> EPGDGAQTWARFSRPPAPEAAGLFQGTFPDGFLWAVGSAAYQTEGGWQQHGKGASIWDTFTHHPLAPPGDSRNASLPLGAPSPLQPATGDVASDSYNNVFRDTEALRELGVTHYRFSISWARVLPNGSAGVPNREGLRYYRRLLERLRELGVQPVVTLYHWDLPQRLQDAYGGWANRALADHFRDYAELCFRHFGGQVKYWITIDNPYVVAWHGYATGRLAPGIRGSPRLGYLVAHNLLLAHAKVWHLYNTSFRPTQGGQVSIALSSHWINPRRMTDHSIKECQKSLDFVLGWFAKPVFIDGDYPESMKNNLSSILPDFTESEKKFIKGTADFFALCFGPTLSFQLLDPHMKFRQLESPNLRQLLSWIDLEFNHPQIFIVENGWFVSGTTKRDDAKYMYYLKKFIMETLKAIKLDGVDVIGYTAWSLMDGFEWHRGYSIRRGLFYVDFLSQDKMLLPKSSALFYQKLIEKNGFPPLPENQPLEGTFPCDFAWGVVDNYIQVDTTLSQFTDLNVYLWDVHHSKRLIKVDGVVTKKRKSYCVDFAAIQPQIALLQEMHVTHFRFSLDWALILPLGNQSQVNHTILQYYRC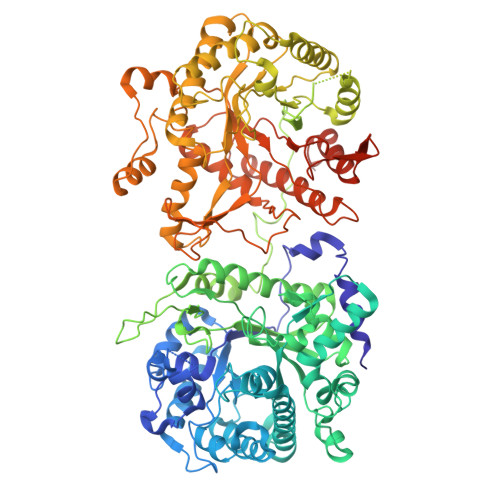MASELVRVNITPVVALWQPMAPNQGLPRLLARQGAWENPYTALAFAEYARLCFQELGHHVKLWITMNEPYTRNMTYSAGHNLLKAHALAWHVYNEKFRHAQNGKISIALQADWIEPACPFSQKDKEVAERVLEFDIGWLAEPIFGSGDYPWVMRDWLNQRNNFLLPYFTEDEKKLIQGTFDFLALSHYTTILVDSEKEDPIKYNDYLEVQEMTDITWLNSPSQVAVVPWGLRKVLNWLKFKYGDLPMYIISNGIDDGLHAEDDQLRVYYMQNYINEALKAHILDGINLCGYFAYSFNDRTAPRFGLYRYAADQFEPKASMKHYRKIIDSNGFPGPETLERFCPEEFTVCTECSFFHTRKSHHHHHH ETHYL 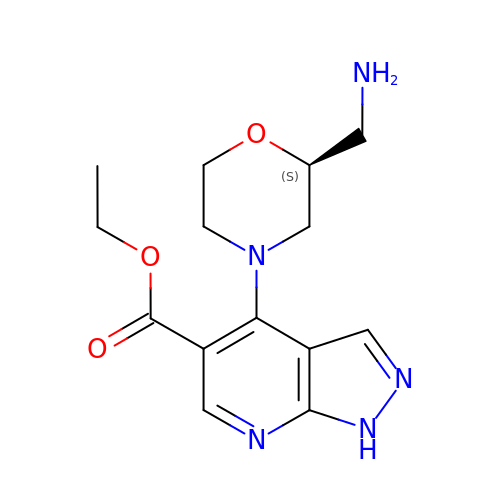4-(2-(AMINOMETHYL)MORPHOLINO)-1H-PYRAZOLO[3,4-B]PYRIDINE-5-CARBOXYLATE | C14 H19 N5 O3 | RCMLOOJGYJFCJA-VIFPVBQESA-N> GEYASVTDVYNYYKYGELLRGGICHSVQLTAAISNGCIKNGKHNIFIIGDSYAAALFNGLSHY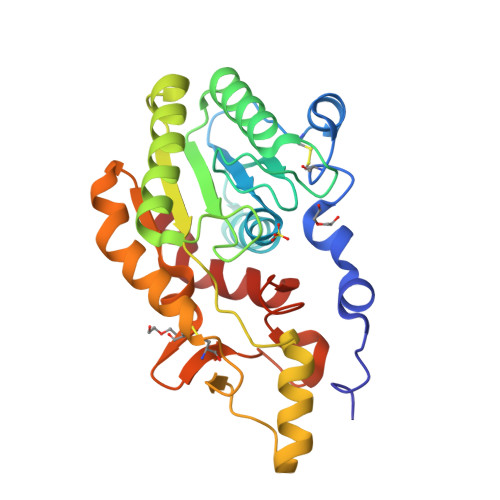IDNKGSDYIISQMTDGNAPPLFVDGKDDLQRSVITLNNNRINEIKRVQPEVVLLTWSVRGTNGVHDKKLAIDALSLTIKKIKEASPDSRIIFIGPVPEWNANLVKIISNYLSEFKKTPPLYMTYGLNSEISEWDSYFSNNVPKMGIEYISAYKALCNESGCLTRVGNGPDFITAVDWGHLTKPGSDFLFNKIGNKIIK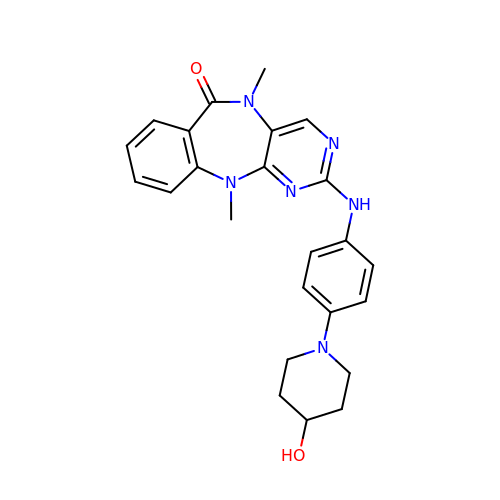2-((4-(4-HYDROXYPIPERIDIN-1-YL)PHENYL)AMINO)-5,11-DIMETHYL-5H-BENZO[E]PYRIMIDO [5,4-B][1,4]DIAZEPIN-6(11H)-ONE | C24 H26 N6 O2 | DFQAJLQXPSPNJE-UHFFFAOYSA-N>[2x]AAGRRGSFVEMVDNLRGKSGQGYYVEMTVGSPPQTLNILVDTGSSNFAVGAAPHPFLHRYYQRQLSSTYRDLRKGVYVPYTQGKWEGELGTDLVSIPHGPNVTVRANIAAITESDKFFINGSNWEGILGLAYAEIARPDDSLEPFFDSL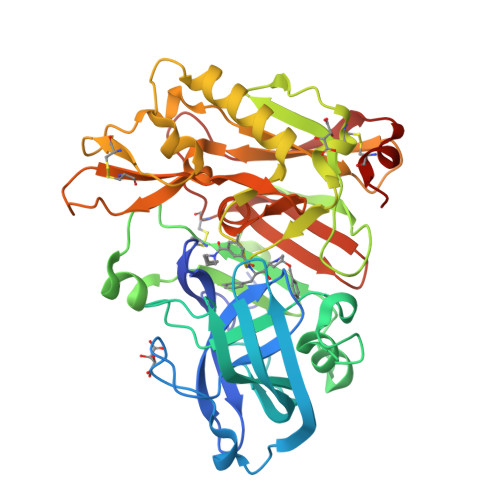VKQTHVPNLFSLQLCGAGFPLNQSEVLASVGGSMIIGGIDHSLYTGSLWYTPIRREWYYEVIIVRVEINGQDLKMDCKEYNYDKSIVDSGTTNLRLPKKVFEAAVKSIKAASSTEKFPDGFWLGEQLVCWQAGTTPWNIFPVISLYLMGEVTNQSFRITILPQQYLRPVEDVATSQDDCYKFAISQSSTGTVMGAVIMEGFYVVFDRARKRIGFAVSACHVHDEFRTAAVEGPFVTLDMEDCGYNI> GGWIRNIGRYLSYLVDDTFEEYAYDVVDGIAKARTQEELLEGVYKALRLAPKLKKKAESKGCPPPRIPSPEDIEALEEKVEQLSNPKDLRKLAVSLALWAFA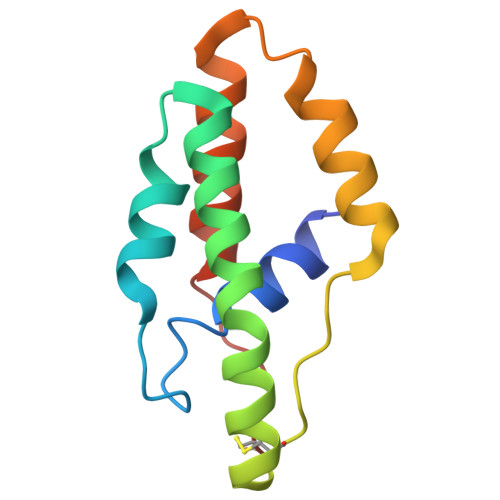SWNNCP>[2x]GHMAPAPPANSGESSLLSESELPAGISYAEAMEGGSRPLLHPDNPVVFFDISIGSHEAGRIKIELFKNLAPKSAENFRQFCTGEFRQNQVPIGYKGATFHR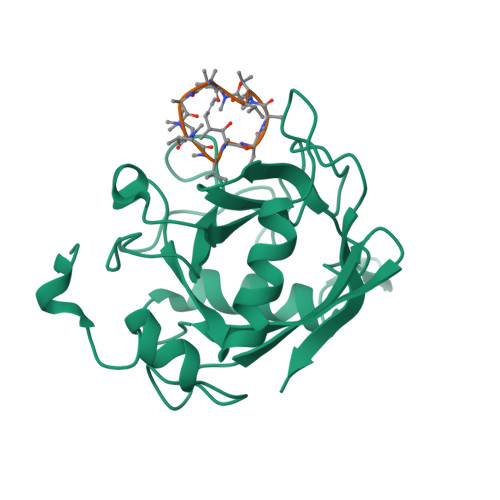IIKNFMIQGGDFVKGDGTGRLSIYGSSFPDEAFVLPHFRSGLLSLANSGPDTNGCQFFITCAKCDWLNRKHVVFGQVLGKESMQVVRKIEHVTVDGGNRPRIPVTVTQCGEL;>ALLVTAAXVLA[2x]> GAMGRMQQQLGRTRSQQEYQQALWYSASAESLALSALSLSLKNEKRVHLEQPWASGPRFFPLPQGQIAVTLRDAQACFNLNALAQPTTASRPLAVQQLIALISR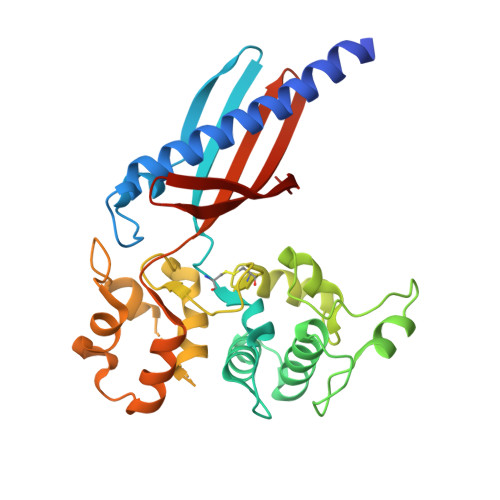LDVPAYRAELIAESLWEFIDEDRSVQTRLGREDSEYLARSVPFYAANQPLADISEMRVVQGMDAGLYQKLKPLVCALPMTRQQININTLDVTQSVILEALFDPWLSPVQARALLQQRPAKGWEDVDQFLAQPLLADVDERTKKQLKTVLSVDSNYFWLRSDITVNEIELTMNSLIVRMGPQHFSVLWHQTGESE>[2x]GAMGPGSDYIIKEKTVLLQKKDSEGFGFVLRGAKAQTPIEEFTPTPAFPALQYLESVDEGGVAWRAGLRMGDFLIEVNGQNVVKVGHRQVVNMIRQGGNTLMVKVVMVTRHPDMDAAAGS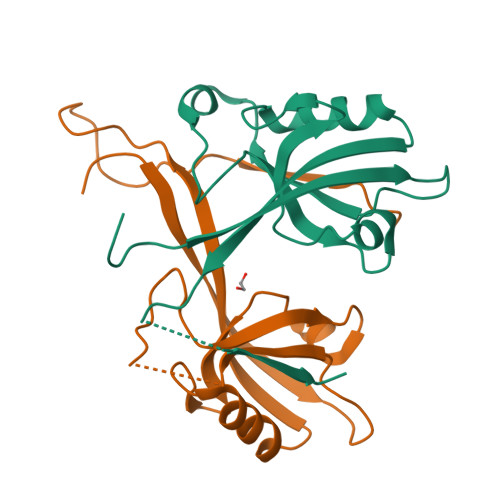GSGSFPELIQDTSTSFSTTR4-(3-phenyl-1,2,4-thiadiazol-5-yl)-N-(pyridin-3-yl)piperazine-1-carboxamide | C18 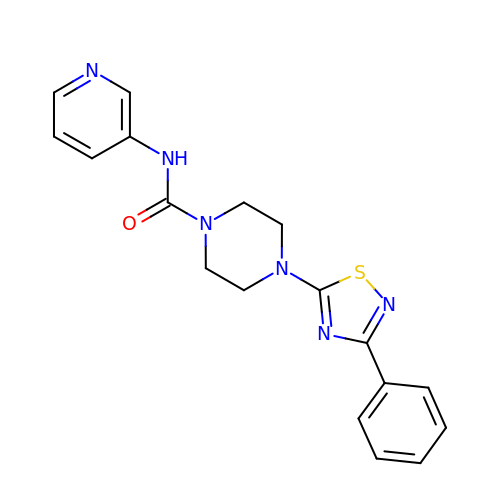H18 N6 O S | RCAFZHFLIBYWGO-UHFFFAOYSA-N> ERPVRVKAWVEENRGSFLPPVCNKLLHQKQLKIMFVGGPNTRKDYHIEEGEEVFYQLEGDMLLRVLERGKHRDVVIRQGEIFLLPAGVPHSPQRFANTVGLVIERRRLKTELDGLRYYVGDTTDVLFEKWFYCEDLGTQLAPIIQEFFSSEQYRTGKPNPDQLLKEPPFPLSTRSVMEPMCLEAWLDGHRKELQAGTPLSLFGDTYESQVMVHGQGSSEGLRRDVDVWLWQLEGSSVVTMEGQRLSL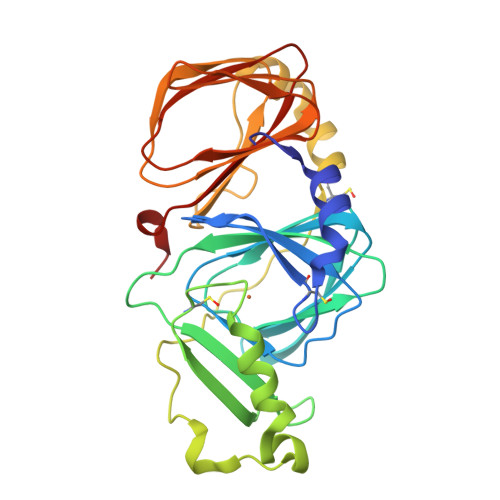TLDDSLLVPAGTLYGWERGQGSVALSVTQDPACKKSLG> MHHHHHHMRMEFRHNLPSSDIIFGSGTLEKIGEETKKWGDKAILVTGKSNMKKLGFLADAIDYLESAGVETVHYGEIEPNPTTTVVDEGAEIVLEEGCDVVVALGGGSSMDAAKGIAMVAGHSAEERDISVWDFAPEGDKETKPITEKTLPVIAATSTSGTGSHVTPYAVITNPETKGKPGFGNKHSFPKVSIVDIDILKEMPPRLTAITGYDVFSHVSENLTAKGDHPTADPLAIRAIEYVTEYLLRAVEDGEDIKAREKMAVADTYAGLSNTISGTTLRHAMAAPISGYYPDISHGQALASISVPIMEHNIENGDEKTWERYSRIAVALDASKPVDNTRQAASKAVDGLKNLLRSLDLDKPLSELGVEEEKIPEMTEGAFIYMG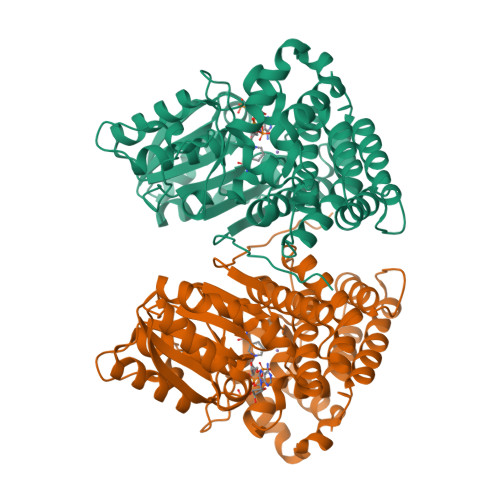GGIEANPVDVSKEDVKEIFRKSL AMINOMETHYLAMIDE | C2 H6 N2 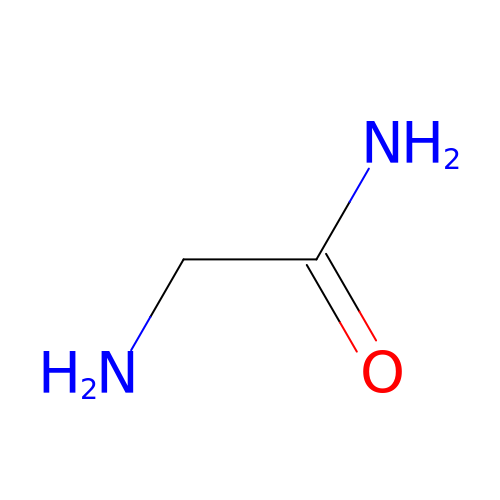O | BEBCJVAWIBVWNZ-UHFFFAOYSA-N> MGRLLRLEVENFKSYRGHQIIGPFEDFTSIIGPNGAGKSNLMDAISFVLGVKSSHLRSTNVKELIYRGKILQRDNTDFTDSSNPTTAYVKLMYELDNGEQREYKRAITPSGATEYKIDEEIVTFSEYCGSLQKENILVRARNFLVFQGDVETIASQSPLELSKLVEQISGSLEYKSEYDKSKDEQDKAVNLSAHSFNKKRGINAELRQYQEQKTEAERYQSQKEKRDSAQLVYLLWKLFHLEKSISSNMAEVTRLKADSIQLIERRDENTKEIEKLKEKEGSIRRNLLAFDRKVRKQEKLIASKRPELISIAEKALESKSNLRKIQRKAAEIEKDYSDQASTLQVLENQLTSLSAAEKEFLKDMQEKEQLKGLRLLPEDKEEYEGLRSEADKLNSNLLFKLQTLNRNIKVTSQSKDSLTSIVGDLESKIKSLHESVSSLDTERADLLAKINEKIESLELEKHDQQKKRLTYSELFHKTQELNEELQSCLQKILEASADRNESKQDAKKREALYALKRIYPEVKGRIIDLCTPTQKKYESAIAAALGKNFDAIVVETQAVAKECIDYIKEQRIGIMTFFPMDTIAASPVNQKFRGTHKGARLAIDVLNFESEYERVMISAVGNTLICDSMTVARDLSYNKRLNAKTVTLEGTVIHKTGLITGGSSNNRSAKHWDDHDFDLLTQTKDRLMHQIGEIEYQKSSCVITESDTVKLHSLESEISLLKDKYTVVSRSVEDKKKEIGHYESLIKEKQPHLSELEMELRNFVKSRDELQIQVEKVEEKIFSGFCKRIGISDIHTYDEIHRTFTQSFTQKQLEFTKQKSLLENRISFEKQRVSDTRLRLERMHKFIEKDQESIDNYEQNREALESEVATAEAELELLKEDFASENSKTEKILLAASEKKLVGKRLVSELTKLSGNITLLESEIDRYVSEWHAILRKCKLEDIDVPLREGSLTSIPIDDVSNSGDITMGEEPSEPVINFEKFGVEVDYDELDEELRNDGSESMASVLQ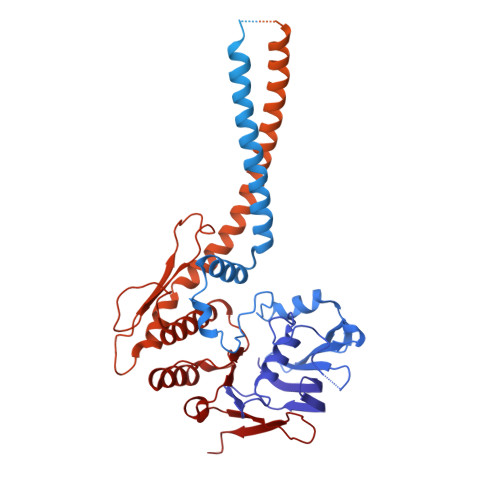EKLREYSEELDQMSPNLRAIERLETVETRLAKLDEEFAAARKAAKNAKERFNAVKQKRLQKFQAAFSHISEQIDPIYKELTKSPAFPLGGTAYLTLDDLDEPYLGGIKFHAMPPMKRFRDMDQLSGGEKTMAALALLFAIHSYQPSPFFVLDEIDAALDQTNVTKIANYIRQHASSGFQFVVISLKNQLFSKSEALVGIYRDQQENSSRTLSINLEGYVE Human T-cell Leukaemia Virus type 1 (HTLV-1) is an untreatable retrovirus that causes lethal malignancies and degenerative inflammatory conditions. Here, we show that high-resolution crystal structures of the mature-length HTLV-1c CA protein define essential lattice interfaces and identify a distinct ligand-binding pocket. Across the known Orthoretrovirinae, CA is a two-domain protein with HIV being the best characterised. However, our structures reveal that HTLV-1 does still have a pocket formed between helices 3, 4, and 5, albeit an electropositive one capable of binding to either phosphate or sulfate in vitro.

During screening, a third crystal form of HTLV-1 CANTD was observed diffracting to 1.47 Å resolution in space group P212121 with two molecules in the asymmetric unit. In this case, the crystallant included 0.2 M ammonium sulfate. In one of the HTLV-1 CANTD molecules, a sulfate ion is unambiguously resolved bound to an electropositive pocket on the NTD surface formed by α-helices 3, 4, 5 and 7. The sulfate ion is coordinated by residues H71, H72, R98, and W117. The sidechains of Q56, H72 and R98 appear to act as gatekeepers that flip up and down to allow the sulfate entry into the pocket. Mutants that would remove a direct interaction with the sulfate or phosphate groups (H71A, H72A, R98A and W117A) all effectively abolished infectivity with a concomitant loss of particle production. As the equivalent site has been exploited for the development of arguably the most potent and longest-acting anti-HIV drug, our structural and phenotype data suggest that similar attention should be paid to this site in HTLV-1 with a view to the development of capsid-targeting pre-exposure prophylactics.

>PVMHPHGVPPSHRPWQMKDLQAIKQEVSQAAPGSPQFMQTIRLAVQQFDPTAKDLQDLLQYLCSSLVASLHHQQLDSLISEAETRGITGYNPLAGPLRVQANNPQQQGLRREYQQLWLTAFAALPGS[2x]>MRKLNPALEFRDFIQVLKDEDDLIEITEEIDPNLEVGAIMRKAYESHLPAPLFKNLKGASKDLFSILGCPAGLRSKEKGDHGRIAHHLGLDPKTTIKEIIDYLLECKEKEPLPPITVPVSSAPCKTHILSEEKIHLQSLPTPYLHVSDGGKYLQTYGMWILQTPDKKWTNWSIARGMVVDDKHITGLVIKPQHIRQIADSWAAIGKANEIPFALCFGVPPAAILVSSMPIPEGVSESDYVGAILGESVPVVKCETNDLMVPATSEMVFEGTLSLTDTHLEGPFGEMHGYVFKSQGHPCPLYTVKAMSYRDNAILPVSNPGLCTDETHTLIGSLVATEAKELAIESGLPILDAFMPYEAQALWLILKVDLKGLQALKTTPEEFCKKVGDIYFRTKVGVLVHEIILVADDIDIFNFKEVIWAYVTRHTPVADQMAFDDVPSFVLAPFVSQSSRSKTMKGGKCVTNCIFRQQYE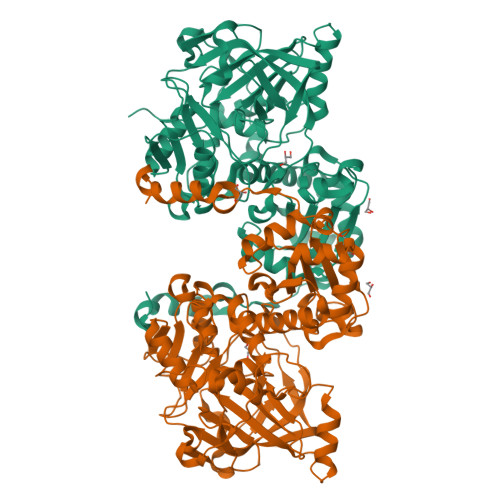RSFDYITCNFEKGYPKGLVDKVNENWKRYGYK[2x]> MTQELGNANFENFIGATEGFSEIAYQFTSHILTLGYAVMLAGLLYFILTIKNVDKKFQMSNILSAVVMVSAFLLLYAQAQNWTSSFTFNEEVGRYFLDPSGDLFNNGYRYLNWLIDVPMLLFQILFVVSLTTSKFSSV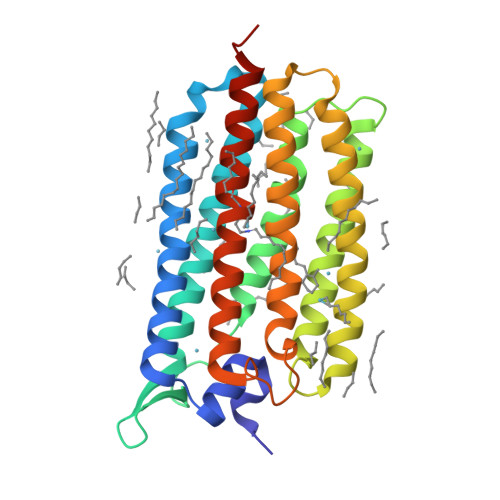RNQFWFSGAMMIITGYIGQFYEVSNLTAFLVWGAISSAFFFHILWVMKKVINEGKEGISPAGQKILSNIWILFLISWTLYPGAYLMPYLTGVDGFLYSEDGVMARQLVYTIADVSSKVIYGVLLGNLAITLSKNKELVEANS> GAMAFNPHTSDLPSSKVNENSLGTLDESKSSDSHSDSDGEQEAEEGGVSTETEKPKIKFKEKNKNSDGGSDPETQKEKSIQKQNSLGSNEEKSKTLKKSNPYGEWQEIKQEVESHEEVDLELPSTENEYVSTSEADGGGEPKVVFKEKTVTSLGVMADGVAPVF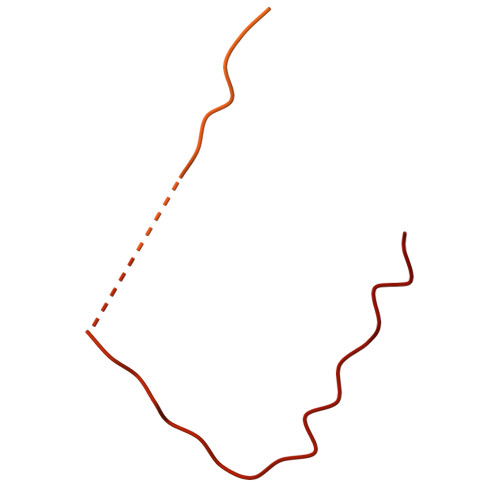KKRRTENGKSRNLRQRGDDQ> MKGLKERQDRRLG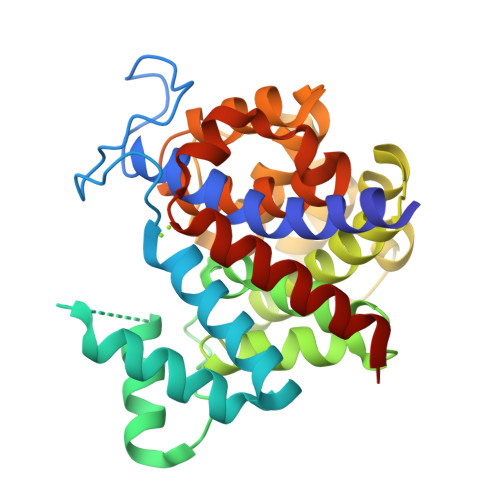AFLGLAVGDALGAQVEGLPKGTFPEVREMKGGGPHRLPPGFWTDDTSQALCLAESLLQRGFDPKDQMDRYLRWYREGYRSATGVCFGLGHATRRALERYAATGDPYAGDEAGAGNGPLMRLAPLVLAYENHPDLLSLARRAARTTHGAREALEATEVLAWLLREALRGAPKEALLALEPFRGADLHPALRRVVEGGFWEAPEEGPGYAPGTLAAALWAFARGRDFEEGMRLAVNLGGDADTVGAVYGQLAGAYYGLGAIPGRWLRALHLREEMEALALALYRMSMASPRE>MGIEYRSLHTSQLTLSEKEALYDLLIEGFEGDFSHDDFAHTLGGMHVMAFDQQKLVGHVAIIQRHMALDNTPISVGYVEAMVVEQSYRRQGIGRQLMLQTNKIIASCYQLGLLSASDDGQKLYHSVGWQIWKGKLFELKQGSYIRSIEEE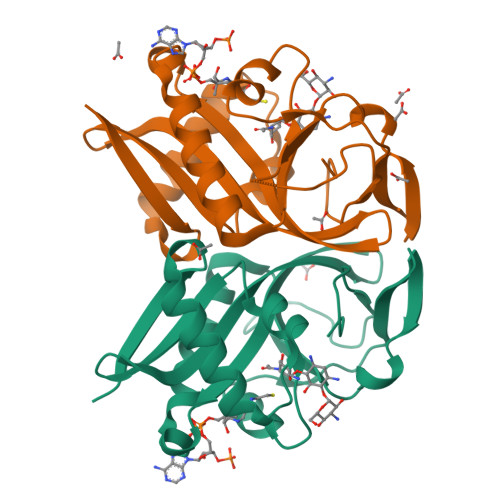GGVMGWKADGEVDFTASLYCDFRGGDQW[2x]> GSHMLSSRISSSDNSSSSTGNEEVRNR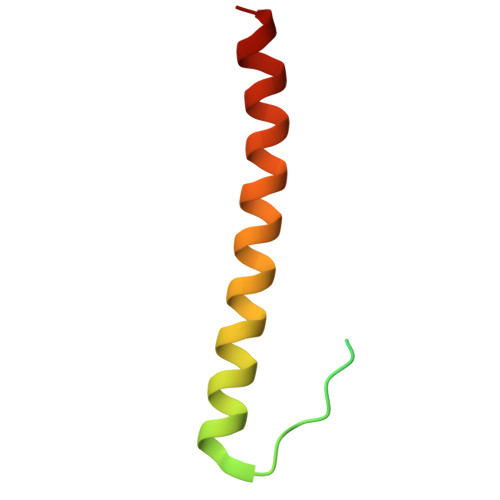SKLPSSKKEREELFRKRKEEMILAARKRMEGKIKGEKQDKN> MEHVAFGSEDIENTLAKMDDGQLDGLAFGAIQLDGD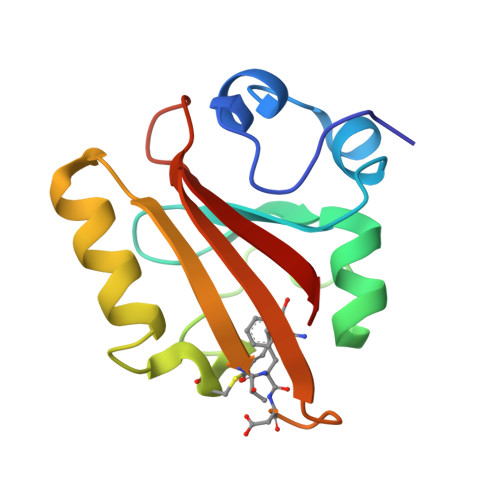GNILQYNAAEGDITGRDPKQVIGKNFFKDVAPCTDSPEFYGKFKEGVASGNLNTMFEYTXDYQMTPTKVKVHMKKALSGDSYWVFVKRV>[2x]MSTAIVTNVKHFGGMGSALRLSEAGHTVACHDESFKHQDELEAFAETYPQLIPMSEQEPVELIEAVTSALGHVDILVSNDIAPVEWRPIDKYAVEDYRDMVEALQIKPFALANAVASQMKRRKSGHIIFITSAASFGPWKELSTYASARAGASALANALSKELGEHNIPVFAIAPNGVDSGDSPYYYPSEPWKTSPEHVAW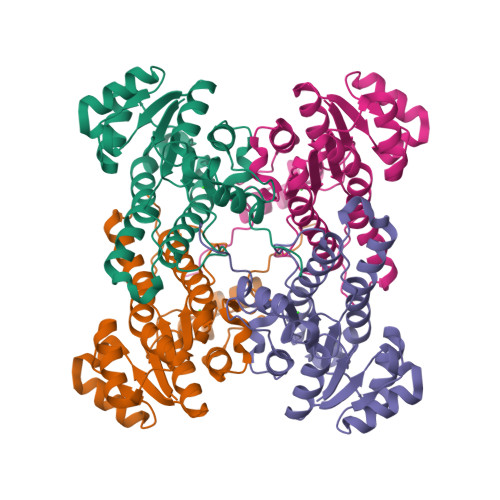VRKYTALQRLGTQKELGELVTFLASGSCDYLTGQVFWLAGGFPVVERWPGMPE7-(4-bromophenyl)-5-phenyl-3,7-dihydro-4H-pyrrolo[2,3-d]pyrimidin-4-one | C18 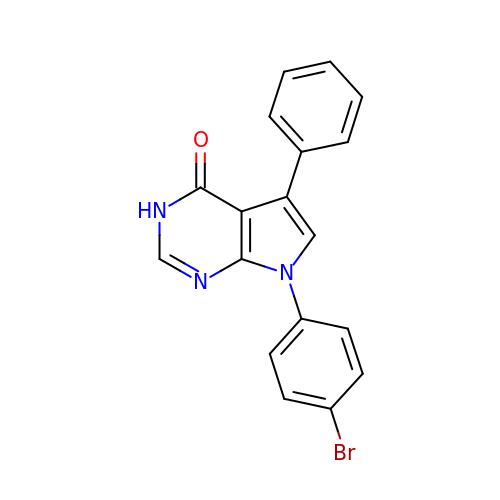H12 Br N3 O | PNDQJUVRRFIFTM-UHFFFAOYSA-N> MASYAELFDIGEDFAAFVGHGLATEQGAVARFRQKLESNGLPSALTERLQRIERRYRLLVAGEMWCPDCQINLAALDFAQRLQPNIELAIISKGRAEDDLRQRLALERIAIPLVLVLDEEFNLL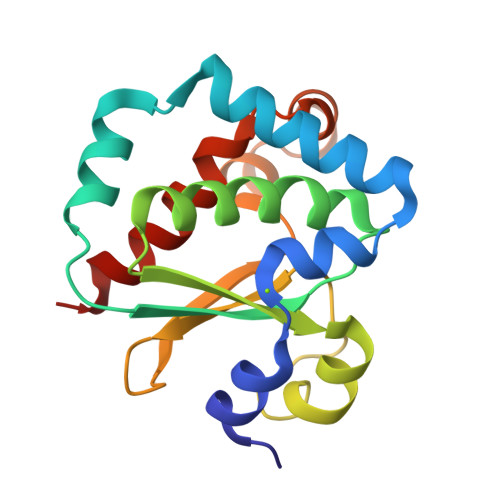GRFVERPQAVLDGGPQALAAYKAGDYLEHAIGDVLAIIEGAAR>SNAMYSMLKRVITEKDLLRQIRLLEQLLNVPQLTAKRLAAQIQTTERTVFSDLQYIRSQLPADWSIETDSSGIRLRNQGNAQTNELWSLFLPQSISIQLLKELLFTKELVTTSFLSTSGVSYETLKRHIKKMNQALRDFHLTIQLTTMTIQLIGAESNIRIFYHRLLVPFTHNNYFFDDYSIHEEHYFQFLKQVYSSELTVETEEIFGACWFFINTIRNKANCRVSQFSFDSKDVLFQLYQPSLAKLYASEGIYLQGEE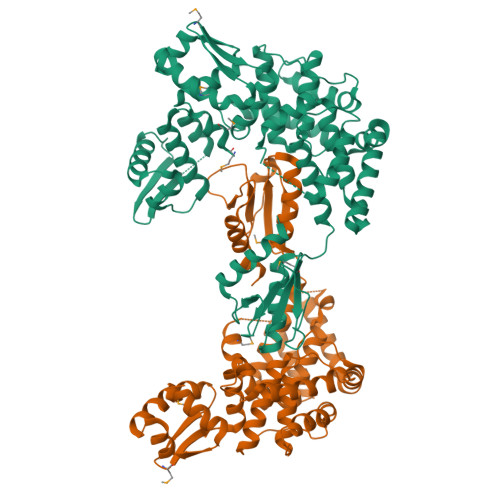SFFAFFCFLESWNYDNVYGETLASALHTHYSQLRKSLQQFVTNLSTEEARPDLIQTNLLDNLLLLFIKYTESPTLSEQFQLEYQELMTEQAAEDLALSKSNQELLEILSRYTTIEEPTYFLSLASLLEKQAIYSIQAQTMTAYFLFQGEPAWKAFLQQELAAYLGTRVKLQAIEYVELSQLTLNEADIIISNFPLDHLDLPVFYLSLIPTKNELRRLAELTLHSYF[2x]> MSGEEERFRAYYERYFAALAARDYETLLEILREFGVAKLVLNGREF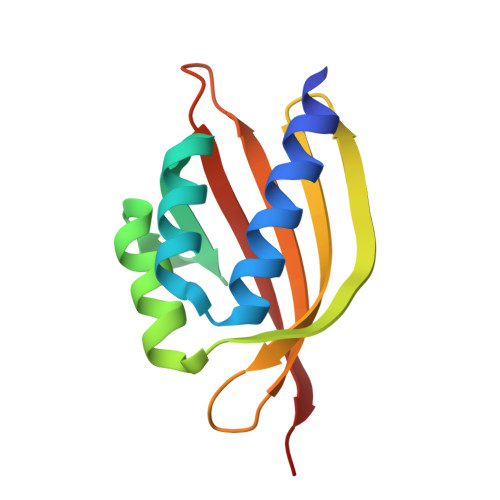ASPEEAVQWARDTGLRFLRLIRERYEDGVYTVEDIVSRDDGRYYRHTSTLRRQPDGSYVQYSQLELLGSG> MGTISSAIINHAFLQNTVMKNCNYKRKRRERDW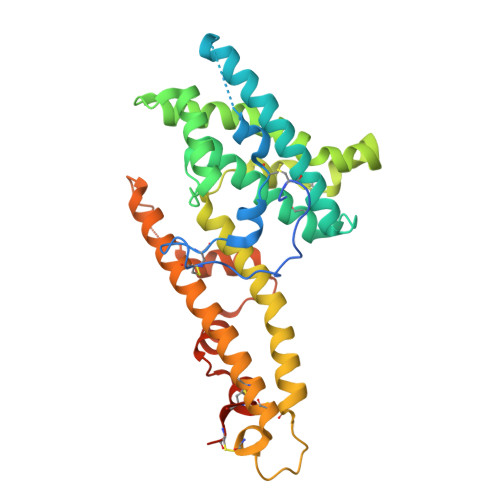DCNTKKDVCIPDRRYQLCMKELTNLVNNTDTNFHRDITFRKLYLKRKLIYDAAVEGDLLLKLNNYRYNKDFCKDIRWSLGDFGDIIMGTDMEGIGYSKVVENNLRSIFGTASTAATSRTSWWNESKAQIWTAMMYSVKKRLKGNFIWICKLNVAVNIEPQIYRWIREWGRDYVSELPTEVQKLKEKCDGKINYTDKKVCKVPPCQNACKSYDQWITRKKNQWDVLSNKFISVKNAEKVQTAGIVTPYDILKQELDEFNEVAFENEINKRDGAYIELCVCSVEEAKKNTQEVVT> QSDLLVPKLTASVTDGAVGVTVDAPVSVTAADGVLAAVTMVNDNGRPVAGRLSPDGLRWSTTEQLGYNRRYTLNATALGLGGAATRQLTFQTSSPAHLTMPYVMPGDGEVVGVGEPVAIRFDENIADRGAAEKAIKITTNPPVEGAFYWLNNREVRWRPEHFWKPGTAVDVAVNTYGVDLGEGMFGEDNVQTHFTIGDEVIATADDNTKILTVRVNGEVVKSMPTSMGKDSTPTANGIYIVGSRYKHIIMDSSTYGVPVNSPNGYRTDVDWATQISYSGVFVHSAPWSVGAQGHTNTSHGSLNVSPSNAQWFYDHVKRGDIVEVVNTVGGTLPGIDGLGDWNIPWDQWRAGNAKA

The essential l,d-transpeptidase of Mycobacterium tuberculosis (LdtMt2) catalyses the formation of 3→3 cross-links in cell wall peptidoglycan and is a target for development of antituberculosis therapeutics. Whereas the d,d-transpeptidases catalyse the formation of 4→3 cross-links between peptidoglycan pentapeptide chains, the functionally related l,d-transpeptidases (Ldts) catalyse the formation of 3→3 cross-links between tetrapeptide chains. The Ldts, which do not manifest structural homology with the PBPs and likely originate from a different evolutionary precursor, share a common YkuD fold (named after the first identified member of this class), distinguished by a β-sandwich with two mixed β-sheets and one helix, and a set of four loops. The established substrate for LdtMt2 is the disaccharide tetrapeptide monomer 1 (GlcNAc-MurNAc-l-Ala-d-iGluNH2-m-DAPNH2-d-Ala).

We were interested in assessing the transpeptidase activity of the active site cysteine to serine mutant of LdtMt2 (LdtMt2C354S), in part because previous reports have shown that in contrast to wild-type LdtMt213,21, LdtMt2C354S is unable to form a covalent complex with several penem and carbapenem derivatives. When LdtMt2C354S was incubated with 1, 2, 3 or 4, no product formation was observed, suggesting the active site cysteine is essential for transpeptidase activity, and cannot be replaced by a potentially nucleophilic serine residue.> KIHTSYDEQSSGESKVKKIEFSKFTVKIKNKDKSGNWTDLGDLVVRKEENGIDTGLNAGGHSATFFSLEEEVVNNFVKVMTEGGSFKTSLYYGYKEEQSVINGIQNKEIITKIEKIDGTEYITFSGDKIK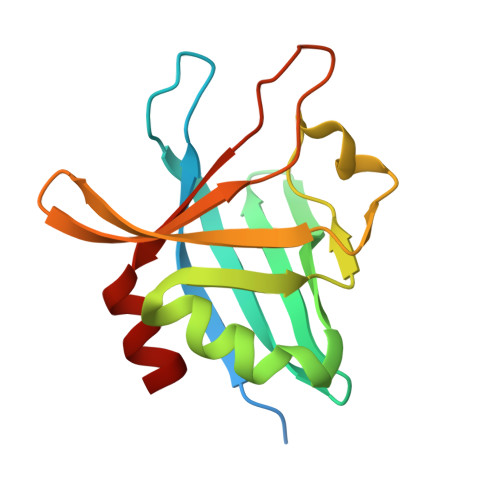NSGDKVAEYAISLEELKKNLK> MEYNF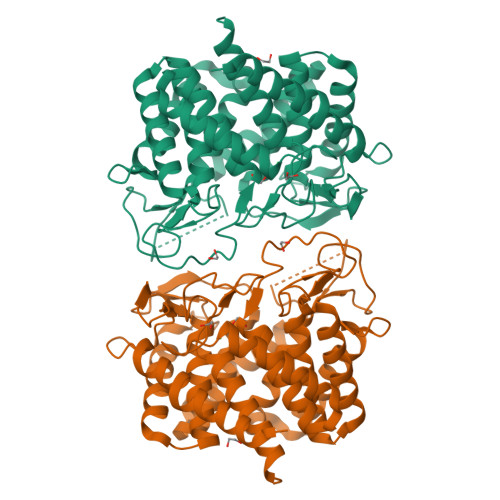QALAELYKNALLNDVLSFWEKYSLDWQQGGYFTCLDREGKIYDTDKFIWLQNRQVWTFSMLYNQLEKRENWLKIASNGANFLAQHGRDSDGNWYFALTREGKPLVHPYNIFSDCFAAMAFSKYALAGGEEWAKDVAMQAYNNVLRRKDNPKGKYNKTYPGTRPMKSLAVPMILANLTLEMEWLLPKETLENVLAETVREVMTDFLDQERGLMYENVAPDGSHIDCFEGRLINPGHGIEAMWFIMDIARRQNDTKTINQAVDVVLNILNFAWDSEYGGLYYFMDADGHPPQQLEWDQKLWWVHLESLVALAMGYRLTGREACWEWYQKMHDYAWSHFADSEYGEWFGYLNRRGEVLLNLKGGKWKGCFHVPRALYLCWQQFEAIATPLQHHHHHH P1-(5'-ADENOSYL)P4-(5'-(2'-DEOXY-THYMIDYL))TETRAPHOSPHATE | C20 H25 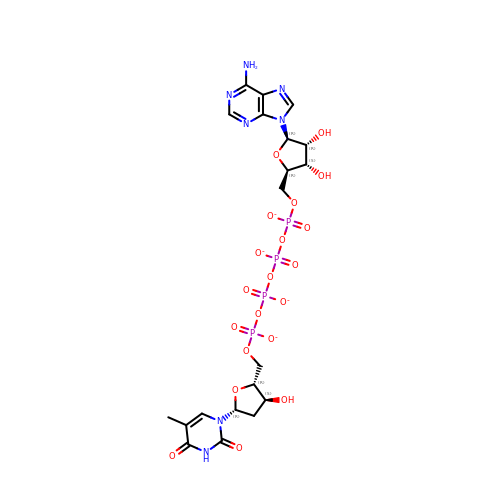N7 O20 P4 | WLGHSSFVEUABFP-SLFMBYJQSA-J>MTEIATTSGARSVGLLSVGAYRPERVVTNDEICQHIDSSDEWIYTRTGIKTRRFAADDESAASMATEACRRALSNAGLSAADIDGVIVTTNTHFLQTPPAAPMVAASLGAKGIL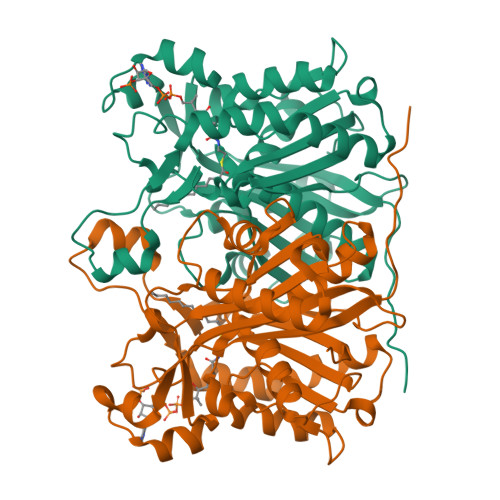GFDLSAGAAGFGYALGAAADMIRGGGAATMLVVGTEKLSPTIDMYDRGNCFIFADGAAAVVVGETPFQGIGPTVAGSDGEQADAIRQDIDWITFAQNPSGPRPFVRLEGPAVFRWAAFKMGDVGRRAMDAAGVRPDQIDVFVPHQANSRINELLVKNLQLRPDAVVANDIEHTGNTSAASIPLAMAELLTTGAAKPGDLALLIGYGAGLSYAAQVVRMPKG[2x]>[12x]KVKVLWDV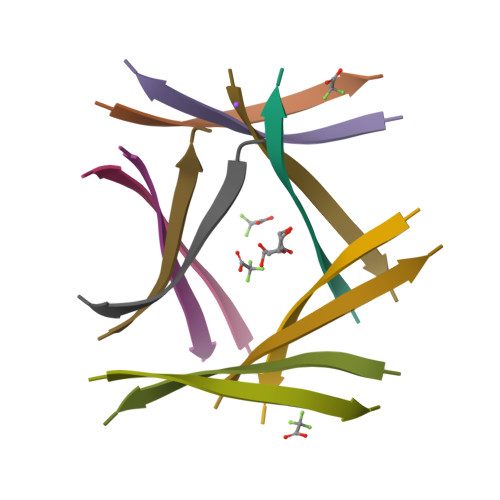IEV> SMQEEDTFRELRIFLRNVTHRLAIDKRFRVFTKPVDPDEVPDYVTVIKQPMDLSSVISKIDLHKYLTVK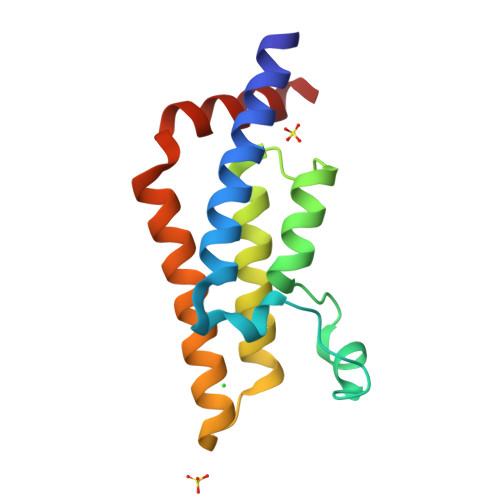DYLRDIDLICSNALEYNPDRDPGDRLIRHRACALRDTAYAIIKEELDEDFEQLCEEIQESR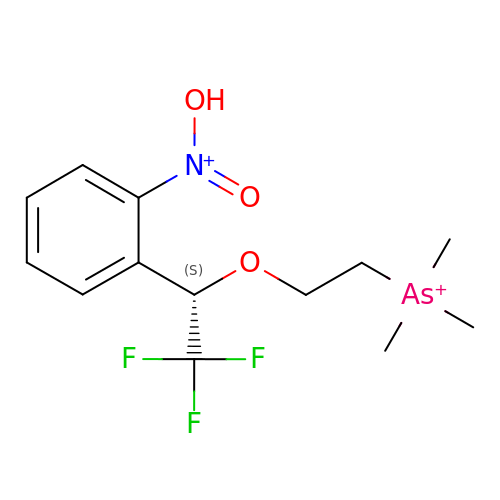1-(2-nitrophenyl)-2,2,2-trifluoroethyl]-arsenocholine | C13 H19 As F3 N O3 | LUSVMAVUPPIHKA-LBPRGKRZSA-N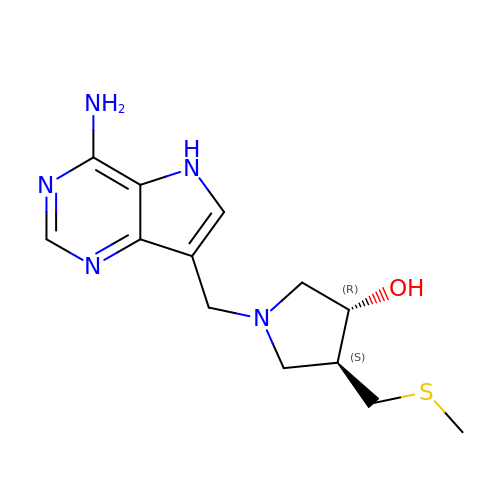(3R,4S)-1-[(4-AMINO-5H-PYRROLO[3,2-D]PYRIMIDIN-7-YL)METHYL]-4-[(METHYLSULFANYL)METHYL]PYRROLIDIN-3-OL | C13 H19 N5 O S | NTHMDFGHOCNNOE-ZJUUUORDSA-N Besides 10–23 DNAzyme, 8–17 DNAzyme can also efficiently catalyze the cleavage reaction of RNA substrate, forming the 5′-product with a 2′,3′-cyclic phosphate at the 3′-end and the 3′-product with a hydroxyl group at the 5′-end; similar structural features are also observed on the cleavage products of the naturally occurred hammerhead, hairpin, and hepatitis delta virus (HDV) ribozymes. Interestingly, the same catalytic motif of 8–17 DNAzyme has been independently isolated under different selection conditions and using different cation cofactors, indicating that this small DNAzyme is efficient and its catalytic core motif is ubiquitous in the sequence space. The central catalytic core of 8–17 DNAzyme is flankedbytwo substrate-recognizing arms, which bind to the RNA substrate via the canonical Watson–Crick base pairing. The Dz36/substrate complexes assemble into a “V” shape with two arms (P1 and P2) orientated ~70° with respect to each other in all the three structures. Unexpectedly, the catalytic core forms a compact small DNA pseudoknot consisting of two short duplexes (P3 and P4) perpendicular to each other.

Two types of non-cleavable 23-nt substrate analogs, including one native DNA and one DNA with 2′-OMe-G at the cleavage site, were utilized in the structural studies. To test whether O2′ could affect the local conformation of the catalytic core and to shed more light on the catalytic mechanism of the DNAzyme, 2′-OMe protection was introduced to the cleavage site (rG-1) of the DNAzyme(2′-OMe-G) structure. Unlike DNAzyme-Pb2+, the DNAzyme(2′-OMe-G) structure belongs to the P43212 space group. Owing to the different molecular packing, the relative orientations of AsfvPolXs are significantly different in the DNAzyme-Pb2+ and DNAzyme-(2′-OMe-G) structures; however, except the blunt-end base pairs that interact with AsfvPolXs, the central regions of the Dz36/substrate complexes are very similar in the two structures, indicated by the low rmsd value (0.586 Å) between them. Although the introduction of the 2′-OMe group did not cause an obvious change to the nucleobase and sugar pucker of G−1 in the DNAzyme-(2′-OMe-G) structure, it led to the shifting of both G13 nucleobase and G+1 phosphate group. When compared to the DNAzyme-Pb2+ structure, the distance (4.3 Å) between the N1 atom of G13 and the OP1 atom of G+1 is 1.5 Å longer in the DNAzyme-(2′-OMe-G) structure. The sugar puckers adopt C2′-endo conformations for G-1 residues in both DNAzyme-(2′-OMe-G) and DNAzyme-Pb2+ structures, whereas the sugar puckers of G+1 residues adopt the C1′-exo and the C3′-endo conformations in the two structures, respectively.

>[2x]GGSMLTLIQGKKIVNHLRSRLAFEYNGQLIKILSKNIVAVGSLRREEKMLNDVDLLIIVPEKKLLKHVLPNIRIKGLSFSVKVCGERKCVLFIEWEKKTYQLDLFTALAEEKPYAIFHFTGPVSYLIRIRAALKKKNYKLNQYGLFKNQTLVPLKITTEKELIKELGFTYRIPKKRL methyl 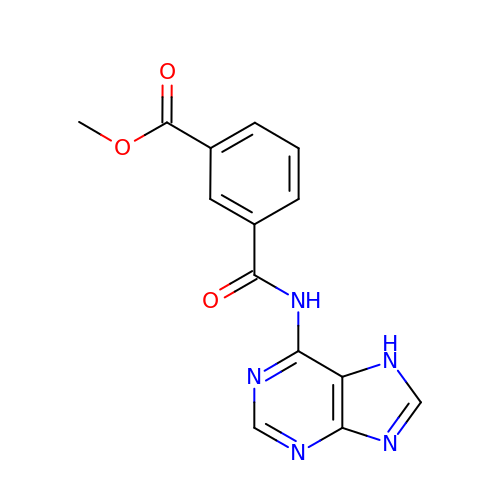3-(7~{H}-purin-6-ylcarbamoyl)benzoate | C14 H11 N5 O3 | NEJKFBOKJSVKCS-UHFFFAOYSA-N2,5-anhydro-1-deoxy-1-phosphono-6-O-phosphono-D-glucitol | C6 H14 O10 P2 | 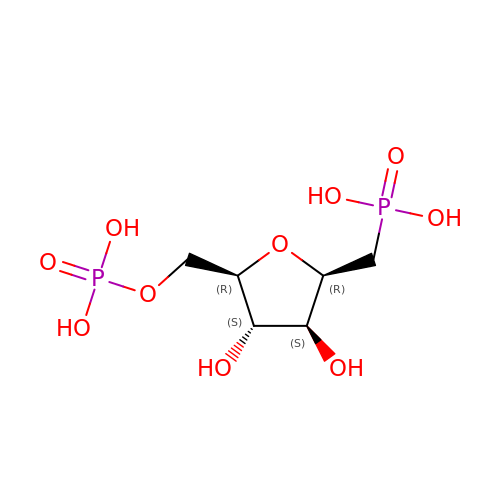YBOWGOLYQKBCFB-JGWLITMVSA-N>MAHHHHHHVDDDDKMRTRSTISTPNGITWYYEQEGTGPDVVLVPDGLGECQMFDSSVSQIA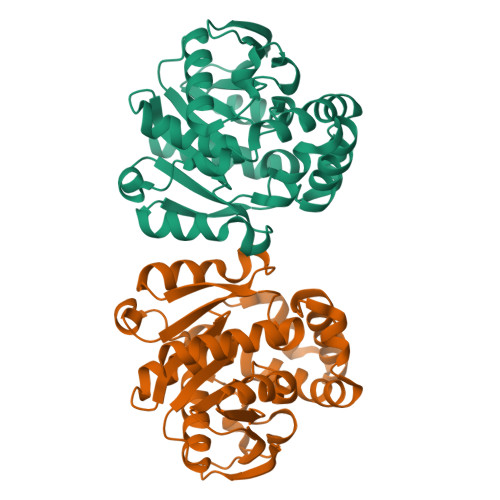AQGFRVTTFDMPGMSRSAKAPPETYTEVTAQKLASYVISVLDALDIKHATVWGCSSGASTVVALLLGYPDRIRNAMCHELPTKLLDHLSNTAVLEDEEISKILANVMLNDVSGGSEAWQAMGDEVHARLHKNYPVWARGYPRTIPPSAPVKDLEALRGKPLDWTVGAATPTESFFDNIVTATKAGVNIGLLPGMHFPYVSHPDVFAKYVVETTQKHL[3x]>GUGAAAGUGUACCUAGGGUUCCAGCCUAUUUGUAGGUGUUCGGACCGAGCGGUACAGGUAUAUUUUUAUAUACCACACCUUAGGGACAAAAGCCCGGGAG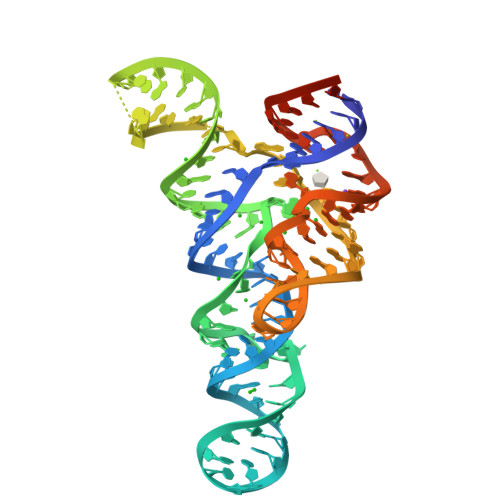GAUAGGUUUCACUCGUA[2x]> GGKKKNKEGSG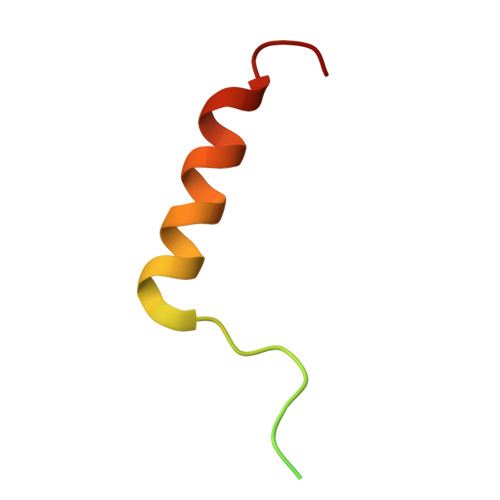DGGRAELNPWPEYIYTRLEMYNILKAEHDSILAE> QECTKFKVSSCRECIESGPGCTWCQKLNFTGPGDPDSIRCDTRPQLLMRGCAADDIMDPTSLAETQEDHNGGQKQLSPQKVTLYLRPGQAAAFNVTFRRAKGYSRVF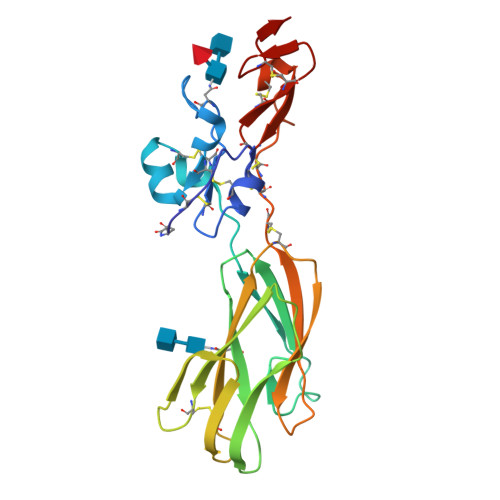LDHNALPDTLKVTYDSFCSNGVTHRNQPRGDCDGVQINVPITFQVKVTATECIQEQSFVIRALGFTDIVTVQVLPQCECRCRDQSRDRSLCHGKGFLECGICRCDTGYIGKNCEHHH D-phenylalanyl-N-[(2S,3S)-6-{[amino(iminio)methyl]amino}-1-chloro-2-hydroxyhexan-3-yl]-L-phenylalaninamide 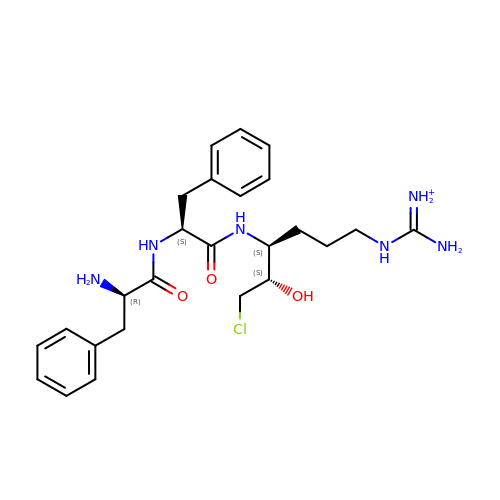| C25 H36 Cl N6 O3 | ZKHBINZTIMXMQW-CLAROIROSA-O> MGSDKIHHHHHHENLYFQGMKKVFITTGTEHYLRQLMENYIGENVTLLQNFSQSLLYQESTGEKLFQEGKEYRVLQSSGSLKGFGIVVFEYIQLRDEEIPIFLQMYQHASLHFSETPGLQSTKLTKAMNTNQFLIVSFWDSE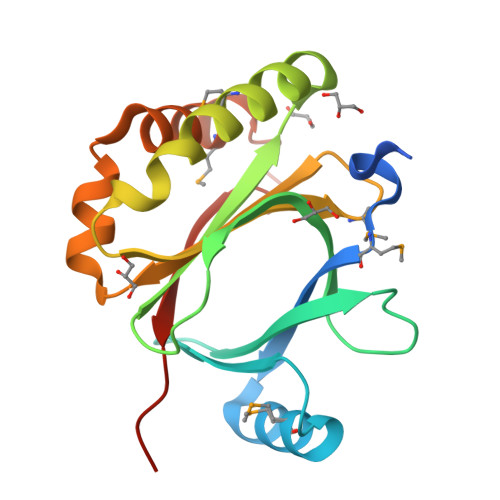VFFQEWKKTPLHKEITSIMKKNNTQVGFSHEDIYHYPEFSHDAK> MVMGIFANCIFC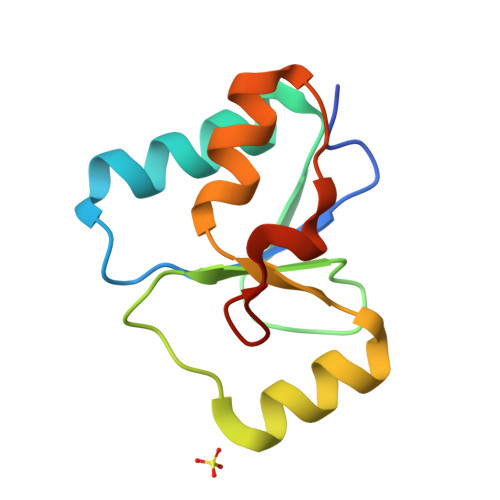LKVKYLPQQQKKKLQTDIKENGGKFSQSLNPQCTHIILDNADVLSQYQLNSIQKNHVHIANPDFIWKSIREKRLLDVKNYDPYKPLDI Identification of SAMHD1 as the factor that impedes infection of myeloid cells by HIV and SIV brought to light an intrinsic cellular antiviral immunity mechanism that relies on controlled reduction of deoxynucleotide triphosphate (dNTP) availability. To counter this infectivity block, HIV-2 and SIV viruses encode an auxiliary protein Vpx, which targets SAMHD1 for proteasomal degradation and facilitates infection of noncycling immune cells by these viruses. In this study, we show that the allosteric binding sites of the enzyme are plastic and can accommodate oligonucleotides in place of the allosteric activators, GTP and dNTP. Collectively, our results shed new light onto the intricate allosteric regulation of SAMHD1 activity and raise questions about the role of nucleic acid phosphorothioation in dNTP metabolism and antiviral immunity in bacteria and in humans.

We then investigated the stereospecificity of the interaction. DNA phosphorothioation replaces one nonbridging oxygen with sulfur and creates a chiral center at phosphorous. Conventional solid-phase synthesis of phosphorothioated oligonucleotides is not stereoselective and the two stereoisomers, Rp and Sp, can occur with roughly equal probability at each phosphorothioate linkage. To further explore this, we used NMR to investigate the interaction of SAMHD1 with the d(TG*TTCA) oligonucleotide containing a single phosphorothioate bond after the sole G nucleotide. This oligonucleotide was used because it could be readily separated into pure Rp and Sp diastereomers by reverse-phase chromatography. When SAMHD1 was titrated into the NMR sample of crude d(TG*TTCA), we observed that 1H NMR signals corresponding to the Rp diastereomer of the oligo gradually disappeared, whereas the signals of the Sp diastereomer were affected to a much lesser degree. Finally, we cocrystallized SAMHD1 with the crude d(TG*TTCA) oligonucleotide and resolved positions of the sulfur atoms in the crystal using anomalous scattering of sulfur in the monochromatic X-ray beam at a long wavelength (1.7712 Å). In the anomalous electron-density map, location of the sulfur atoms in the SAMHD1/ d(TG*TTCA) complex corresponded to the Rp stereoisomer. Furthermore, when the oligonucleotide was modeled without the phosphorothioate modification (e.g., oxygen modeled in place of sulfur), a significant positive difference map peak appeared at the Rp position to indicate the presence of the larger sulfur scatterer. In summary, the recognition of the GpsN modification by SAMHD1 is stereospecific for the Rp conformation of the phosphorothioate linkage.

>MWSHPQFEKGSGSENLYFQGGGGGKVINDPIHGHIELHPLLVRIIDTPQFQRLRYIKQLGGGYYVFPGASHNRFEHSLGVGYLAGCLVHALGEKQPELQISERDVLCVQIAGLCHDLGHGPFSHMFDGRFIPLARPEVKWTHEQGSVMMFEHLINSNGIKPVMEQYGLIPEEDICFIKEQIVGPLESPVEDSLWPYKGRPENKSFLYEIVSNKRNGIDVDKWDYFARDCHHLGIQNNFDYKRFIKFARVCEVDNELRICARDKEVGNLYDMFHTRNSLHRRAYQHKVGNIIDTMITDAFLKADDYIEITGAGGKKYRISTAIDDMEAYTKLTDNIFLEILYSTDPKLKDAREILKQIEYRNLFKYVGETQPTGQIKIKREDYESLPKEVASAKPKVLLDVKLKAEDFIVDVINMDYGMQEKNPIDHVSFYCKTAPNRAIRITKNQVSQLLPEKFAEQLIRVYCKKVDRKSLYAARQYFVQWCADRNFTKPQDGDVIAPLITPQKKEWNDSTSVQNPTRLREASKSRVQLFKDDPM[4x]> MENQLFIIGIGTGTDEYENFEETILKGVKRNELEGQIGPDILDNCCSDVCYFWGRSKETIYEKKIDKGDMVLFYVGKRISRNKVDLNQETAVYLGIICETVEISENDVSF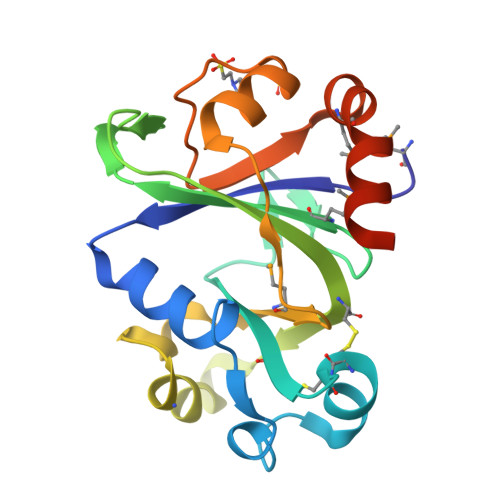LNDFWRKGENFRFLMFFKKKPEKLHHSINEINSKLGYNPDYFPIAGYVKPERMSGVYDILKNILKKRGILKESDS> MDGSGEQPRGGGPTSSEQIMKTGALLLQGFIQDRAGRMGGEAPE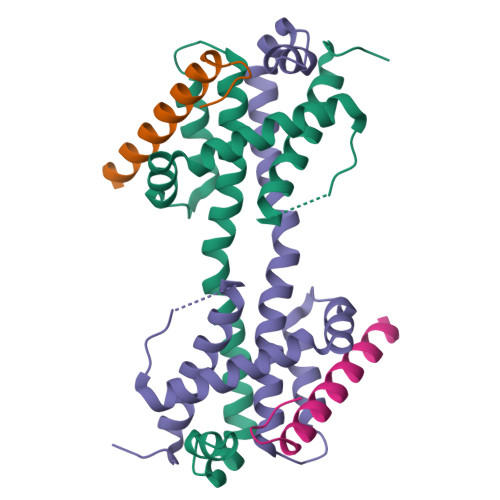LALDPVPQDASTKKLSESLKRIGDELDSNMELQRMIAAVDTDSPREVFFRVAADMFSDGNFNWGRVVALFYFASKLVLKALSTKVPELIRTIMGWTLDFLRERLLGWIQDQGGWDGLLSYFGTPTWQGSS;> SESQEDIIRNIARHLAQVGDSMDRSIPPGLVNGL(3S)-1-(3-aminocarbonylphenyl)carbonyl-2,3-dihydroindole-3-carboxylic 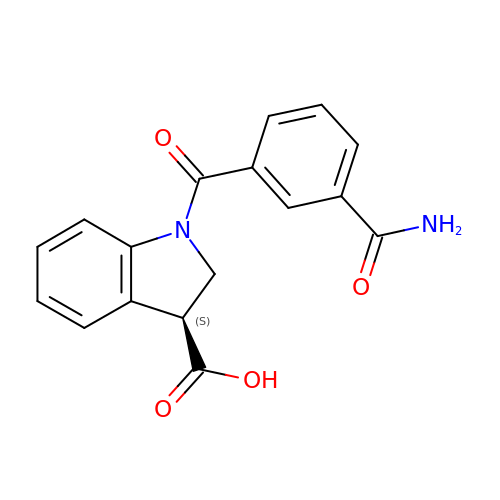acid | C17 H14 N2 O4 | OYXRIJPFODLVER-CYBMUJFWSA-N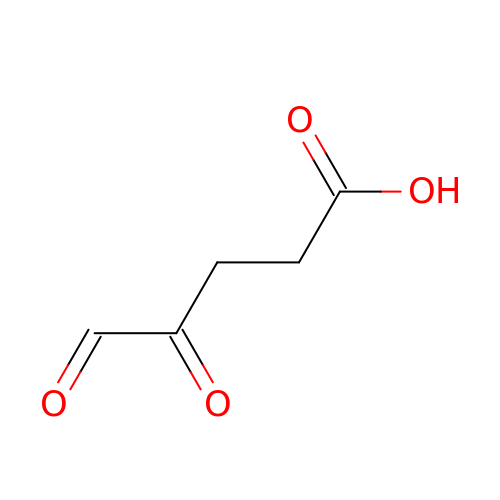4,5-DIOXOPENTANOIC ACID | C5 H6 O4 | YHUFRVYVNKGICT-UHFFFAOYSA-N> MNILKHFPSYVGPSKIRTLVIPIGHWTRKEFNNAVQKLSEFNEIHLSDVTPIDSPIFTPQGFPHGKLFFDFLTIDHDDALELFLYDFEPFRKTFVIIGLVNDYSDPLTNLNFMKEKYPTLISPNLVYASSTPTKELEQTIDTMENVFASSPDMQKNIETIMCDIARNFLTALNSYYSSYKHVTLRSPGAIGGNAVLKTTLIRQNSYTSSSSSTPMSAVQSSVSSSSKAGSVTTASKRLSSFEMTTNSLKRSASLKLATTLSTSENRSQQKSLGRQMKILGNFQLLAGRYVDALNSFVDAITTLYKVRDYLWLGSALDGISICFLLLSYLGLSYQIPQIVSLICPVEKLNFESSSTGISPVDSNSKATASTTASSTPRNSISIAAMQSPRNSIMSLSAPALNIDVENINLPLLIKCISDKVLYYYDLSLMHNSEYAPQVVYCEFLLKTLTFMTSCYKSSEFSKDVLDNIVKNQHRALSDIPNSPMFPRFEVYFYSNKLFELQLKEMQVEAQIKIYSTMAEVYRLLGYKRKQLFVLRLLMVALLATPNKIAWHPDYRTLIDTIIELLNINESEAKINVDDPSQSTWLILQKK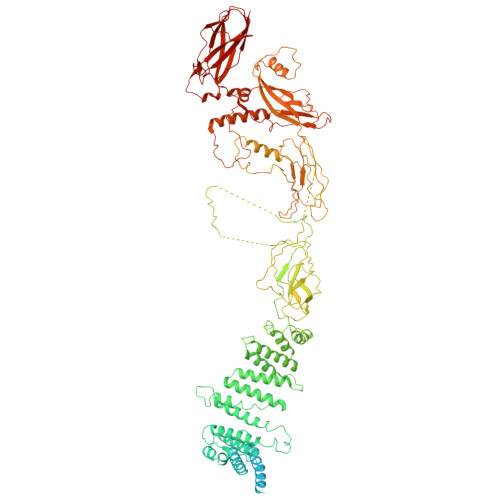ILQLCIKVSRKINDFEYVAKFSSILITKYTHLLNQSEQDALFKEYIQPSITNESITSYWDPFILREVVINRILDSDPTSNEIPLESDVSSLESLENRQKTQDINPQEVFNPFKRVQPTSFVSNNSTKVPILVFLVGDKAEFTCRVQNPFKFDFTINDIQLDEEISEFCEIDRKAVSYSGPYNVKAESIRSITLPLIIKKPTYKKIYEISCLKISILKLPLQKFDIINDSRRSNPVEEEAEYSKCIYGKLKIKILPEQPQLELLSTSKMTRNSWMMLDGTKTDFHITVRNKSLSCAINHIKIIPMNNIEQMLKPDYWKKMPPDDLYIMEKQLDWLSKSCVRIIKLPTVIKPNETITFDLELDNTAVPFNFTGFDLLIEYGMSATDESCIYLKKLSIPYEVTLRRTIEVPSMDIIPLNELFSSQVENVDWIEYVMSKIRAESNLHSRDFILLLLDFRNSWIDGIKLNVQFEDFTSNEYHVEASHTSRIIVPIKKIDYKKYNFENTPIPRIFPGRQFIQSGLNEEQTIEMRQKFWCREHIISKLKCNWKLTTDQSVTGSVDFNKFIEKFDHKMVYTIYPGRLFYGVQLLLDEPKVKVGEIINLKIITEPTSTCRRKQNSTVNFLDIVIFDSKTSKILPRSNRRILYNGSLTKPISTTKVSEINLEIIPIEKGRYEFSVCISKSNNQDGIIQFDSENVILSVI> GMASVLSAATATDQGPVRENNQDACLADGILYAVADGFGARGHHASATALKTLSAGFAAAPDRDGLLEAVQQANLRVFELLGDEPTVSGTTLTAVAVFEPGQGGPLVVNIGDSPLYRIRDGHMEQLTDDHSVAGELVRMGEI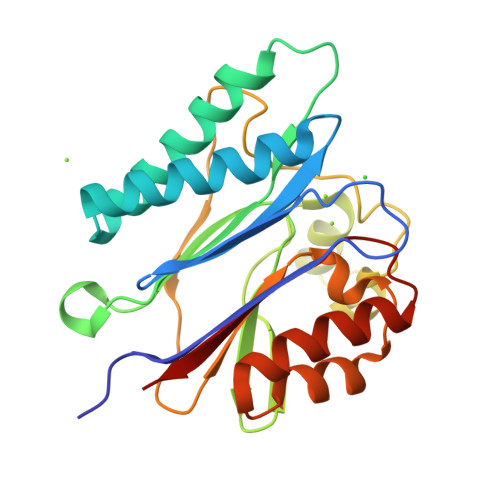TRHEARWHPQRHLLTRALGIGPHIGPDVFGIDCGPGDRLLISSDGLFAAADEALIVDAATSPDPQVAVRRLVEVANDAGGSDNTTVVVIDLG>[2x]MSFTPANRAYPYTRLRRNRRDDFSRRLVRENVLTVDDLILPVFVLDGVNQRESIPSMPGVERLSIDQLLIEAEEWVALGIPALALFPVTPVEKKSLDAAEAYNPEGIAQRATRALRERFPELGIITDVCLDPFTTHGQCGILDDD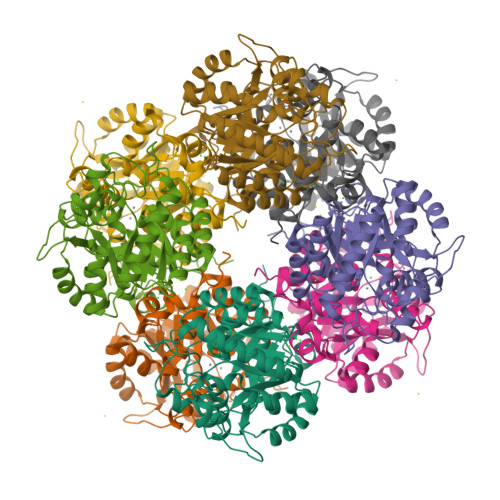GYVLNDVSIDVLVRQALSHAEAGAQVVAPSDMMDGRIGAIREALESAGHTNVRVMAYSAKYASAYYGPFRDAVGSASNLGKGNKATYQMDPANSDEALHEVAADLAEGADMVMVKPGMPYLDIVRRVKDEFRAPTFVYQVSGEYAMHMGAIQNGWLAESVILESLTAFKRAGADGILTYFAKQAAEQLRRGR> MANFMIYPISKDLKNGNSELVRVYSKSKEIQYIKIYTKKIINPGTTEEYEVDIPNWDGGLVVTPQKVILPAGASKSIRLTQF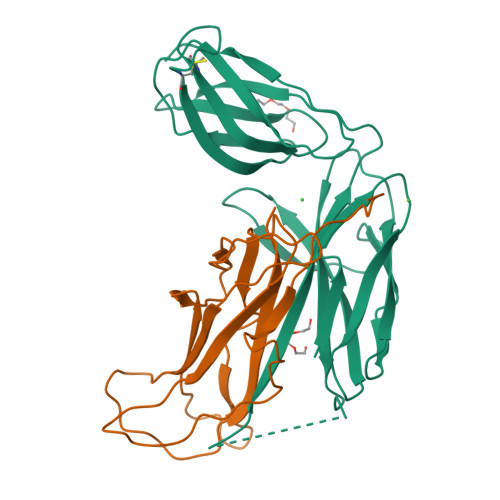KIPKKEEVYRVYFEAVKPDSKENVIDNKKLTIELSVNIIYAALIRSLPSEQNISLNISRNAKKNIIIYNNGNVRAGVKDIYFCKSSNIDDNCVKKAYNKNIYPEKSFDTLVNNNFSYVFIKLNHEGIEKEQGLIQLKVPAAWSHPQFEK;> MVHHHHHHVIDLLQADGNALPSAVKLAYSPASKTFESYRVMTQVHTNADAKKVIVKLADTPQATDVLNSTVQMPISVSWGGQVLSTTAKEFEAAALGYSASGVNGVSSSQELVISAAPKTAGTAPTAGNYSGVVSLVMTLGS> AAQTNAPWGLARISSTSPGTSTYYYDESAGQGSCVYVIDTGIEASHPEFEGRAQMVK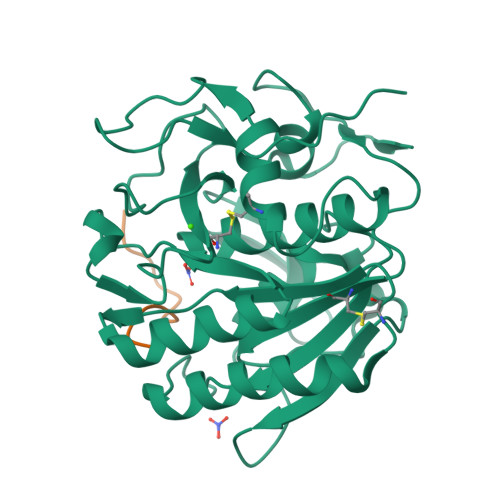TYYYSSRDGNGHGTHCAGTVGSRTYGVAKKTQLFGVKVLDDNGSGQYSTIIAGMDFVASDKNNRNCPKGVVASLSLGGGYSSSVNSAAARLQSSGVMVAVAAGNNNADARNYSPASEPSVCTVGASDRYDRRSSFSNYGSVLDIFGPGTDILSTWIGGSTRSISGTSMATPHVAGLAAYLMTLGKTTAASACRYIADTANKGDLSNIPFGTVNLLAYNNYQA;> KLKLLVVIRLK>MIVSAIAANALLESVTKFHCGVIYDYSTAEYVSYRPSDFGAYLDALEAEVARGGLIVFHNGHKYDVPALTKLAKLQLNREFHLPRENCIDTLVLSRLIHSNLKDTDMGLLRSGKLPGKRFGSHALEAWGYRLGEMKGEYKDDFKRMLEEQGEEYVDGMEWWNFNEEMMDYNVQDVVVTKALLEKLLSDKHYFPPEIDFTDVGYTTFWSESLEAVDIEHRAAWLLAKQERNGFPFDTKAIEELYVELAARRSELLRKLTETFGSWYQPKGGTEMFCHPRTGKPLPKYPRIKTPKVGGIFKKPKNKAQREGREPCELDTREYVAGAPYTPVEHVVFNPSSRDHIQKKLQEAGWVPTKYTDKGAPVVDDEVLEGVRVDDPEKQAAIDLIKEYLMIQKRIGQSAEGDKAWLRYVAEDGKIHGSVNPNGAVTGRATHAFPNLAQIPGVRSPYGEQCRAAFGAEHHLDGITGKPWVQAGIDASGLELRCLAHFMARFDNGEYAHEILNGDIHTKNQIAAELPTRDNAKTFIYGFLYGAGDEKIGQIVGAGKERGKELKKKFLENTPAIAALRESIQQTLVESSQWVAGEQQ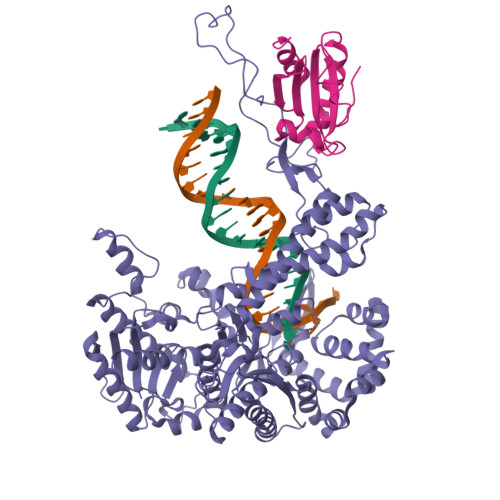VKWKRRWIKGLDGRKVHVRSPHAALNTLLQSAGALICKLWIIKTEEMLVEKGLKHGWDGDFAYMAWVHDEIQVGCRTEEIAQVVIETAQEAMRWVGDHWNFRCLLDTEGKMGPNWAICH[2x];>SDKIIHLTDDSFDTDVLKADGAILVDFWAEWCGPCKMIAPILDEIADEYQGKLTVAKLNIDQNPGTAPKYGIRGIPTLLLFKNGEVAATKVGALSKGQLKEFLDANLA[2x]> SNQLQQLQNPGESPPVHPFVAPLSYLLGTWRGQGEGEYPTIPSFRYGEEIRFSHSGKPVIAYTQKTWKLESGAPMHAESGYFR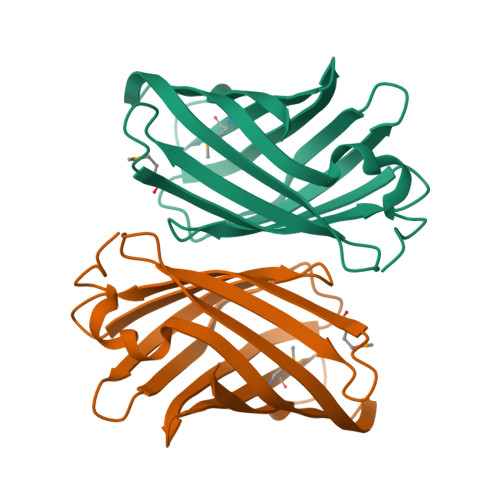PRPDGSIEVVIAQSTGLVEVQKGTYNVDEQSIKLKSDLVGNASKVKEISREFELVDGKLSYVVRMSTTTNPLQPHLKAILDKL DICLOSAN | C12 H8 Cl2 O2 | 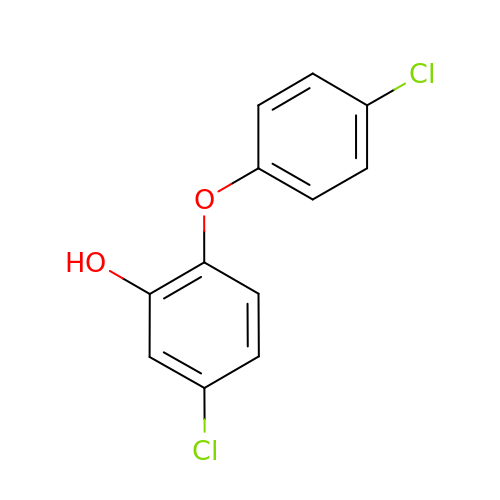BYNQFCJOHGOKSS-UHFFFAOYSA-N Poaceae species use a unique chelation strategy, whereby plants secrete a high-affinity metal chelator, known as phytosiderophores (mugineic acids), and reabsorb the iron-phytosiderophore complex by the yellow stripe 1/yellow stripe 1-like (YS1/YSL) transporter for efficient uptake of iron from the soil. Here, we present three cryo-electron microscopy structures of barley YS1 (HvYS1) in the apo state, in complex with an iron-phytosiderophore complex, Fe(III)-deoxymugineic acid (Fe(III)–DMA), and in complex with the iron-bound synthetic DMA analog (Fe(III)–PDMA). The structures reveal a homodimeric assembly mediated through an anti-parallel β-sheet interaction with cholesterol hemisuccinate. HvYS1 comprises two distinct domains: a substrate-binding YS core and a scaffold domain, implicating an elevator-like transport.

The cryo-EM map was reconstructed to an overall resolution of 2.9 Å with an imposed C2 symmetry. The structure of HvYS1 reveals a homodimeric structure. Four CHS molecules within the HvYS1 dimer are assigned, and two of them are present between the protomers (see also “Dimer interface”). The first 47 residues and the linker between TM6 and TM7 were invisible owing to their flexibilities. The N- and C-halves in the scaffold domain are pinned through a disulfide bond between Cys250 and Cys671. The overall structure of the HvYS1 protomer represents an outward open conformation, as the central cavity is wide open to the extracellular space, whereas the base of the cavity is sealed from the cytoplasm. The scaffold domains from each protomer comprise the dimer interface with a buried surface area of 936 Å2. Each protomer’s C-terminal β -strands (S1s) form an anti-parallel β-sheet to assemble the dimer. In addition, a cluster of the hydrophobic residues including Phe240 and Tyr244 on TM4, Phe252 and Phe255 in the TM4–H4 loop, Phe271 in the H4–H5 loop, Met672 and Phe674 on S1, pack together to stabilize the dimer. The side chain of Tyr451 in the apo structure points inside to occupy the Fe(III)–DMA binding site.

>[2x]MDIVAPDRTRIAPEIDRDEALEGDRESDPALASTREWQLEDMPRWQDELTVRGLVAALLIGFIYTVIVMKIALTTGLVPTLNVSAALLSFLALRGWTRLLERFGVVSRPFTRQENTIVQTCGVACYTIAFAGGFGSTLLGLNKKTYELAGDSPGNVPGSWKEPGIGWMTGFLLACSFGGLLTLIPLRQVLVVDYKLVYPSGTATAILINGFHTDQGDKNSRKQIRGFLKYFGGSFLWSFFQWFYTGGDACGFVQFPTFGLKAWKQTFYFDFSMTYVGAGMICPHIVNISTLLGAIISWGIMWPLISKNKGDWYPAKVPESSMKSLYGYKAFICIALIMGDGMYHFIKIVGITAMSMYRQFSHKQVNNKAKNADDTVSLEELHRQEIFKRGHIPSWMAYAGYALFSVLAVVTIPVMFKQVKWYYVVIAYVVAPMLGFANSYGTGLTDINMGYNYGKIALFVFAGWAGKENGVIAGLVAGTLVKQLVLISADLMQDFKTSYLTQTSPKSMMIAQVVGTAMGCIVSPLTFMLFYKAFDIGNPDGTWKAPYALIYRNMAILGVEGFSVLPKYCIVISGGFFAFAAILSITRDVMPHKYAKYVPLPMAMAVPFLVGGSFAIDMCLGSLIVFAWTKINKKEAGFMVPAVASALICGDGIWTFPASILALAKIKPPICMKFLPAATSAAHHHHHHHH> AQSVPWGISRVQAPAAHNRG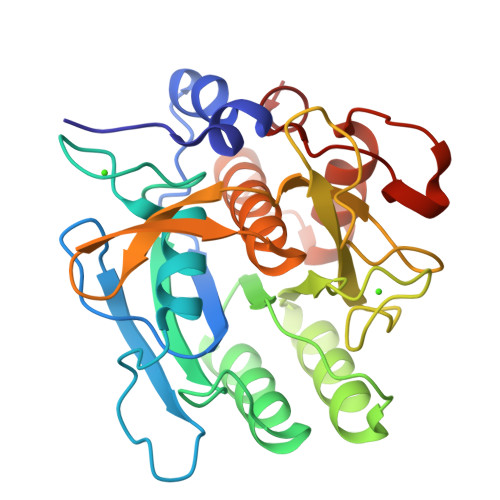LTGSGVKVAVLDTGISTHPDLNIRGGASFVPGEPSTQDGNGHGTHVAGTIAALNNSIGVLGVAPNAELYAVKVLGASGGGSNSSIAQGLEWAGNNGMHVANLSLGSPSPSATLEQAVNSATSRGVLVVAASGNSGAGSISYPARYANAMAVGATDQNNNRASFSQYGAGLDIVAPGVNVQSTYPGSTYASLNGTSMATPHVAGAAALVKQKNPSWSNVQIRNHLKNTATSLGSTNLYGSGLVNAEAATR Ene-reductases (ERs) from the family of the Old Yellow Enzyme (OYE; E.C. 1.6.99.1) are nicotinamide-dependent flavoproteins catalyzing the asymmetric hydrogenation of a wide panel of activated alkenes (e.g., α,β-unsaturated ketones, aldehydes, nitroalkenes, carboxylic acids, and derivatives). We selected a new thermophilic ene-reductase homologue in Chloroflexus aggregans, a peculiar filamentous bacterium. We report here on the functional and structural characterization of this new enzyme, which we called CaOYE. Produced in high yields in recombinant form, it proved to be a robust biocatalyst showing high thermostability, good solvent tolerance and a wide range of pH optimum.

CaOYE was solved and refined in C2221 orthorhombic space group, with 4 molecules per ASU. The overall structure of CaOYE shows the typical α8/β8 TIM barrel fold described till now, for all OYEs reported. The enzyme accommodates one molecule of FMN cofactor on the top of the β-barrel core, at the C-terminus side, buried within the active site cavity (for further details). In agreement with the general behavior of Class III OYEs, crystal contacts support a dimeric architecture, despite native gel analysis and size exclusion chromatography suggesting the protein behaves as a monomer in solution (respectively). The interaction surface between monomers in the functional dimer covers 1451 Å2. The two monomers interact via at least 8 salt bridges. As already reported for the other described Class III OYEs, the C-terminus of each monomer stretches through an “Arg finger” (in our case Arg352) reaching the active site of the adjacent monomer, interacting with the respective flavin cofactor and vice versa. The difference electronic density map Fo–Fc shows an elongated organic molecule, most likely malonate, present within the crystallization precipitant agents, lying above the isoalloxazine ring of FMN. In the complex with malonate, one carboxylate oxygen of the compound forms a hydrogen bond with the side chains of His177 but not with His180. The other carboxylate moiety of malonate is involved in a network of hydrogen bonding interactions with Tyr28, Cys25 and Arg352 of the adjacent monomer that explores the active site, suggesting a role for all these residues in substrate bonding and positioning.

>[4x]MQPHLFTPLTIGSVTLRNRIGMSPMCQYSAVDGFPTDWHLMHLGARAAGGVGLIILEATAVSPEGRISPFDLGIWSDDHIAALSRIVKLIESLGAVAGIQLAHAGRKASVGRPWEGGKPIAPANGGWPVVGPTAEPFAPGYPTPIPLDAAGIARVVADFATATKRARAAGFRWIEIHAAHGYLLHNFLSPLGNDRNDEYGGDLRGRVRLLSEVTAAVRAEWPSDLPLAVRLSCSDWTPEGLTIADTVEVARMLREQGVDLIDCSSGGIAPGITIPVGEGYQVPFAAQVRREANIATAAVGLITRPEHADAIVRNGDADLVLLGRELLRDPHWPLRAARALGHDLAPPPQYLRAW> MPTTVLYHGDQLGPRPLVILDHSVARLEQSATAVLDACQEAAKRYEAMLSSLAWDHGAVFVPLQVSIG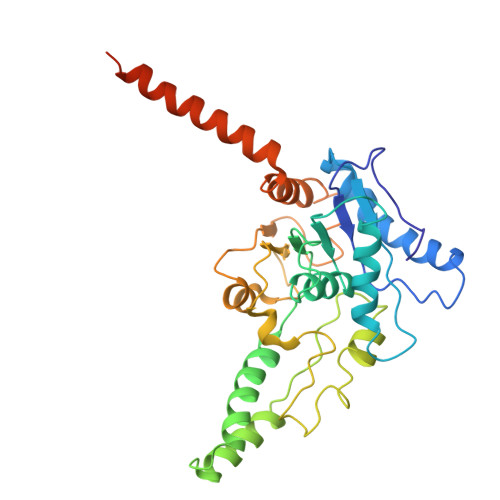EINVMEQSCRHVCAVLDAMDVQWSHVLAHSYGALVAARMAASTAYPHRIGSLLLLDTPLVTEQLVRNTKQREEIAKAKKDVNVPPAELSFAIESLRSALETTLPYPAAVDKSLYEDHLFSSASVFREKGLVRDEHRYVPVRHLAQVHHPLQLLVPVKQPITDVAIHREFFGLRRPAVIKTADNHEDLFSAKCADEVADVVRAWMQRFEPDVVMKRRFEKAAKEMVQLMGSSASFGEKGGGNIEKSEKKEKRKGRQ(5S)-5-methyl-5-[(3-phenyl-1,2-oxazol-5-yl)methyl]pyrrolidine-2,4-dione | 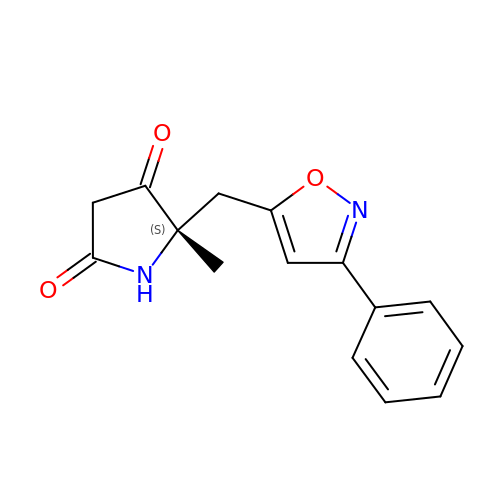C15 H14 N2 O3 | QYMOUPYIBHTJEC-HNNXBMFYSA-N>[2x]SKPIDVSRLDLRIGCIITARKHPDADSLYVEEVDVGEIAPRTVVSGLVNHVPLEQMQNRMVILLCNLKPAKMRGVLSQAMVMCASSPEKIEILAPPNGSVPGDRITFD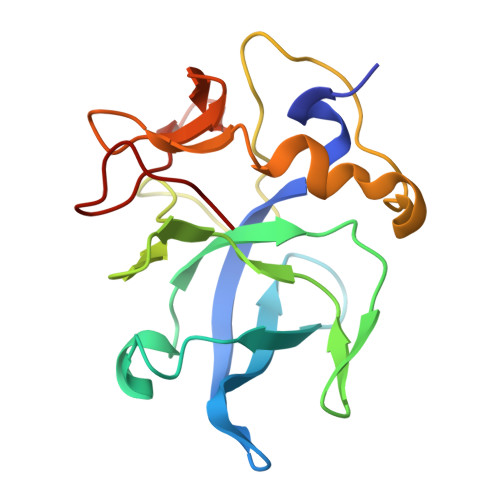AFPGEPDKELNPKKKIWEQIQPDLHTNDECVATYKGVPFEVKGKGVCRAQTMSNSGIK> MAHHHHHHMDLGIAGKTALVCAASKGLGRGCAEALAAEGVNLVIVARTRDTLEETAEEIRA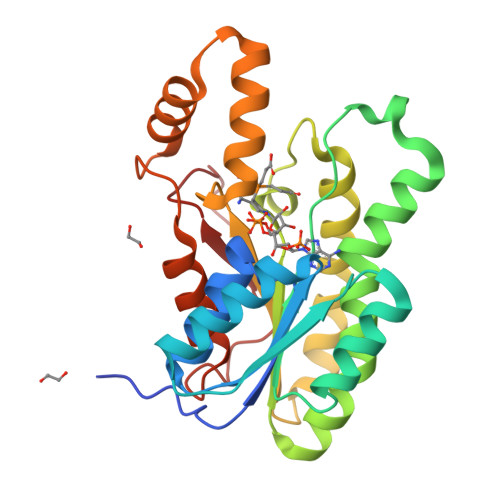ASNVSVTAVACDITTPDGRAAALAACPQPDILVNNAGGPPPGDFRDFSHDDWIRALEANMLTPIELIRATVDGMIGRGFGRIVNITSSAVKAPIDVLALSNGARSGLTGFVAGLSRKVAGQGVTINNLLPGLFDTDRIATTLAASAKAQGVTVDELRARRAKEIPAGRLGTRAEFGAACAFLCSVHAGYITGQNWLLDGGAYPGTF4-{[6-(cyclohexylmethyl)pyridine-2-carbonyl]amino}-3-{[3-(trifluoromethoxy)phenyl]amino}benzoic acid | C27 H26 F3 N3 O4 | 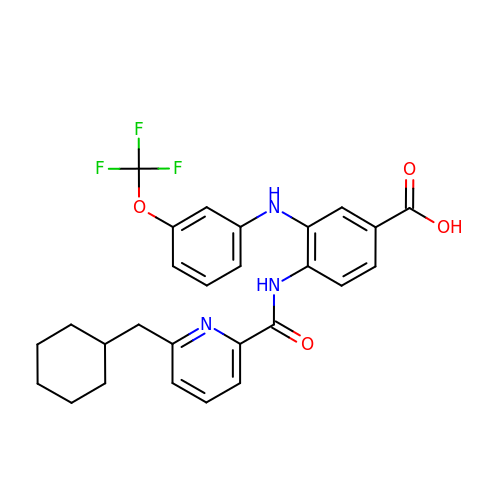OQQHKPTYNRWLGC-UHFFFAOYSA-N>MGHHHHHHHHSSGENLYFQGSKLEFMEGKTRTAPQGEAAGTATTASVPGTTTDGMDPGVVAATSVVTAENSSASVATAGIGGPPQQVDQQETWRTNFYYNDVFTWSVADAPGSILYTVQHSPQNNPFTAVLSQMYAGWAGGMQFRFIVAGSGVFGGRLVAAVIPPGIEIGPGLEVRQFPHVVIDARSLEPVTITMPDLRPNMYHPTGDPGLVPTLVLSVYNNLINPFGGSTNAIQVTVETRPSDDFEFVMIRAPS[2x]

The etiological agent of RHD is rabbit hemorrhagic disease virus (RHDV), which has a single-stranded, positive-sense, polyadenylated RNA genome of ∼7.5 kb. Mature RHDV virions are spherical, non-enveloped particles with a T = 3, icosahedral capsid whose outer diameter varies between 32 and 44 nm and whose structure is defined by characteristic, cup-shaped depressions. The only capsid protein present in RHDV, VP60, is composed of three domains, which include the N-terminal arm (NTA), the shell (S), and the protrusion (P), the latter of which is further divided into P1 and P2 sub-domains.

In this study, we used cryoEM methods to reconstruct the structure of the RHDV capsid to an overall estimated resolution limit of 6.5 Å (5.5 Å in the shell domain) and solved the crystal structures of the S and P domains of the RHDV VP60 protein both at 2.0 Å resolution. The crystal structures of the S and P domains of VP60 were docked into the high-resolution cryoEM map to construct a pseudo-atomic model of the complete RHDV capsid.> MAKYYNEPCHTFNEYLLIPGLSTVDCIPSNVNLSTPLVKFQKGQQSEINLKIPLVSAIMQSVSGEKMAIALAREGGISFIFGSQSIESQAAMVHAVKNFKAGFVVSDSNVKPDQTFADVLAISQRTTHNTVAVTDDGTPHGVLLGLVTQRDYPIDLTQTETKVSDMMTPFSKLVTAHQDTKLSEANKIIWEKKLNALPIIDDDQHLRYIVFRKDYDRSQVCHNELVDSQKRYLVGAGINTRDFRERVPALVEAGADVLCIDSSDGFSEWQKITIGWIREKYGDKVKVGAGNIVDGEGFRYLADAGADFIKIGIGGGSICITREQKGIGRGQATAVIDVVAERNKYFEETGIYIPVCSDGGIVYDYHMTLALAMGADFIMLGRYFARFEESPTRKVTINGSVMKEYWGEGSSRARNWQRYDLGGKQKLSFEEGVDSYVPYA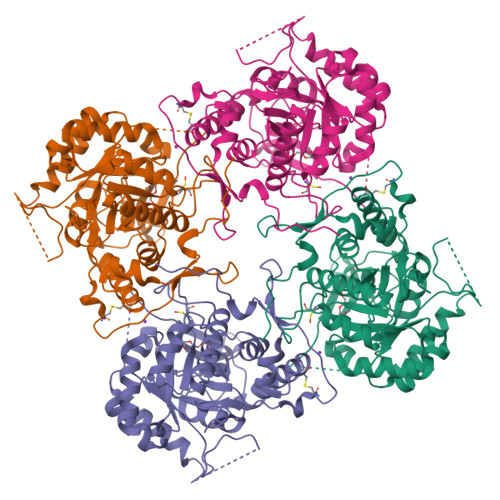GKLKDNVEASLNKVKSTMCNCGALTIPQLQSKAKITLVSSVSIVEGGAHDVIVKDRINDYHPK> MSDPIRTKPKSSMQIDNAPTPHNTPASVLNPSYLKNGNPVRAQAQEQDDKIGTINEEDILANQPLLLQSIQDRLGSLVGQDSGYVGGLPKNVKEKLLSLKTLQSE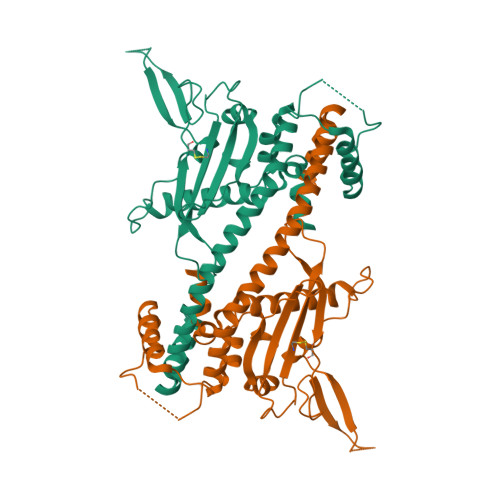LFEVEKEFQVEMFELENKFLQKYKPIWEQRSRIISGQEQPKPEQIAKGQEIVESLNETELLVDEEEKAQNDSEEEQVKGIPSFWLTALENLPIVCDTITDRDAEVLEYLQDIGLEYLTDGRPGFKLLFRFDSSANPFFTNDILCKTYFYQKELGYSGDFIYDHAEGCEISWKDNAHNVTVDLEMRKQRNKTTKQVRTIEKITPIESFFNFFDPPKIQNEDQDEELEEDLEERLALDYSIGEQLKDKLIPRAVDWFTGAALEFEFEEDEEEADEDEDEEEDDDHGLEDDDGESAEEQDDFAGRPEQAPECKQS>[2x]IGTGFPFDPHYVEVLGERMHYVDVGPRDGTPVLFLHGNPTSSYVWRNIIPHVAPTHRCIAPDLIGMGKSDKPDLGYFFDDHVRFMDAFIEALGLEEVVLVIHDWGSALGFHWAKRNPERVKGIAFMEFIRPIPTWDEWPEFARETFQAFRTTDVGRKLIIDQNVFIEGTLPMGVVRPLTEVEMDHYREPFLNPVDREPLWRFPNELPIAG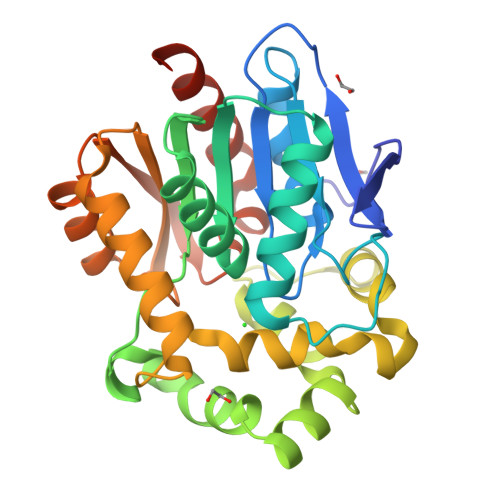EPANIVALVEEYMDWLHQSPVPKLLFWGTPGVLIPPAEAARLAKSLPNCKAVDIGPGLNLLQEDNPDLIGSEIARWLSTLEISGLEHHHHHH>MSDSPVDLKPKPKVKPKLERPKLYKVMLLNDDYTPREFVTVVLKAVFRMSEDTGRRVMMTAHRFGSAVV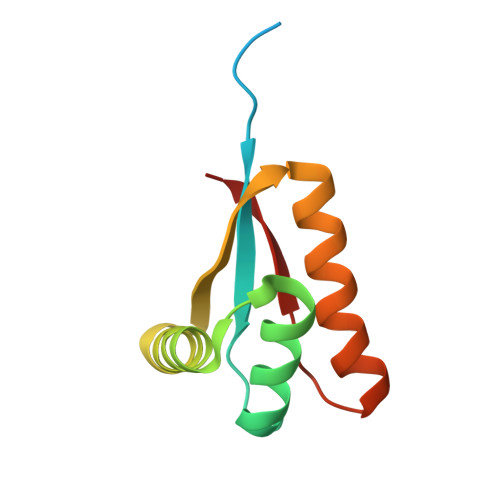VVCERDIAETKAKEATDLGKEAGFPLMFTTEPEE[4x]>[2x]MSLQLLRNTRIFVSTVKTGHNKTNTQEILVQDDISWGQDSNSTDITVNEAGPRPTRGSKRFNDSLNAAEWSFSTYILPYKDKNTSKQIVPDYMLWHALSSGRAINLEGTTGAHNNATNFMVNFKDNSYHELAMLHIYILTDKTWSYIDSCQINQAEVNVDIED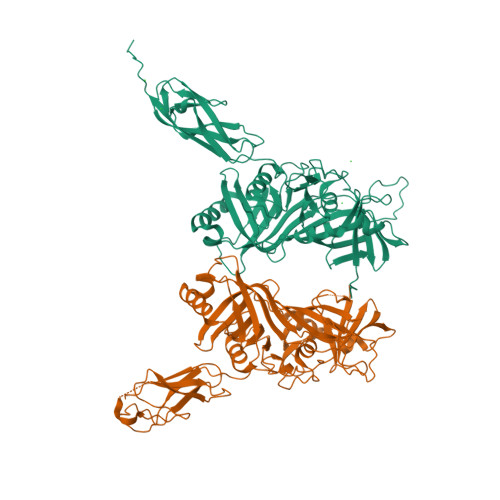IGRVTWSGNGNQLIPLDEQPFDPDQIGIDDETYMTIQGSYIKNKLTILKIKDMDTNKSYDIPITGGTFTINNNITYLTPNVMSRVTIPIGSFTGAFELTGSLTAYLNDKSLGSMELYKDLIKTLKVVNRFEIALVLGGEYDDERPAAILVAKQAHVNIPTIETDDVLGTSVEFKAIPSDLDAGDEGYLGFSSKYTRTTINNLIVNGDGATDAVTAITVKSAGNVTTLNRSATLQMSVEVTPSSARNKEVTWAITAGDAATINATGLLRADASKTGAVTVEATAKDGSGVKGTKVITVTAGGENLYFQGHHHHHH> MHHHHHHSRPKLVTWMNNQRVGELTKL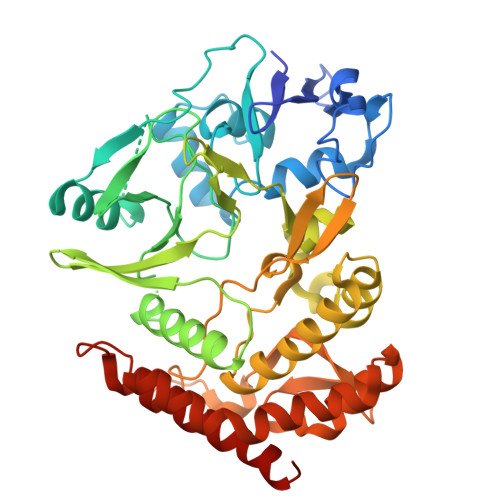ANGAHTFKYAPEWLASRYARPLSLSLPLQRGNITSDAVFNFFDNLLPDSPIVRDRIVKRYHAKSRQPFDLLSEIGRDSVGAVTLIPEDETVTHPIMAWEKLTEARLEEVLTAYKADIPLGMIREENDFRISVAGAQEKTALLRIGNDWCIPKGITPTTHIIKLPIGEIRQPNATLDLSQSVDNEYYCLLLAKELGLNVPDAEIIKAGNVRALAVERFDRRWNAERTVLLRLPQEDMCQTFGLPSSVKYESDGGPGIARIMAFLMGSSEALKDRYDFMKFQVFQWLIGATQGHAKNFSVFIQAGGSYRLTPFYDIISAFPVLGGTGIHISDLKLAMGLNASKGKKTAIDKIYPRHFLATAKVLRFPEVQMHEILSDFARMIPAALDNVKTSLPTDFPENVVTAVESNVLRLHGRLSREYGSK> GAMDDIDEEDDDLVGVSVRPKVPLRTMSYKLAIDMSHFIKEKGGLEGIYYSARRHRILDIYLEKEEGIIPDWQDYTSGPGIRYPKTFGWLWKLVPVNVSDEAQE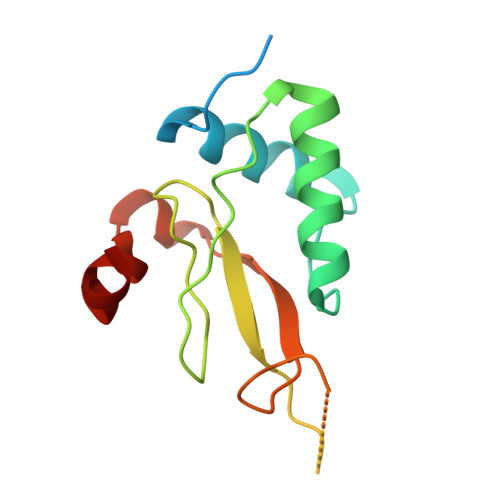DEEHYLMHPAQTSQWDDPWGEVLAWKFDPTLAYTYEAYVRYPEEFGS>HHHHHHNAMQGIHFRRHYVRHLPKEVSQNDII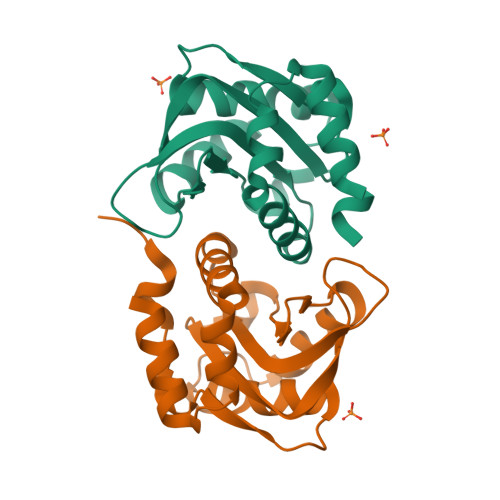KALASPLINDGMVVSDFADHVITREQNFPTGLPVEPVGVAIPHTDSKYVRQNAISVGILAEPVNFEDAGGEPDPVPVRVVFMLALGNWFDITNVLWWIMDVIQDEDFMQQLLVMNDDEIYQSIYTRISE[2x]ISOASCORBIC ACID | C6 H8 O6 | 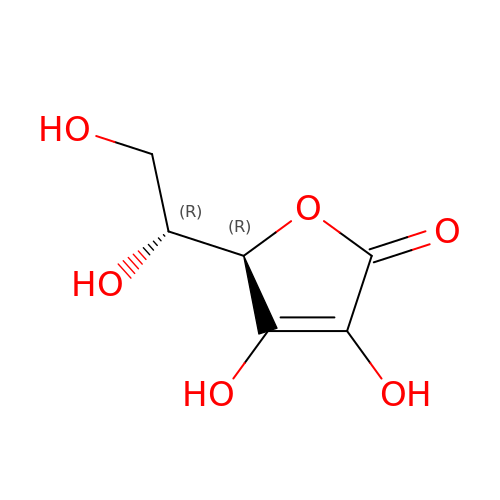CIWBSHSKHKDKBQ-DUZGATOHSA-N>GPQDPYEINLMEELTLKGVTQYYAYVTERQKVHCLNTLFSRLQINQSIIFCNSSQRVELLAKKISQLGYSCFYIHAKMRQEHRNRVFHDFRNGLCRNLVCTDLFTRGIDIQAVNVVINFDFPKLAETYLHRIGRSGRFGHL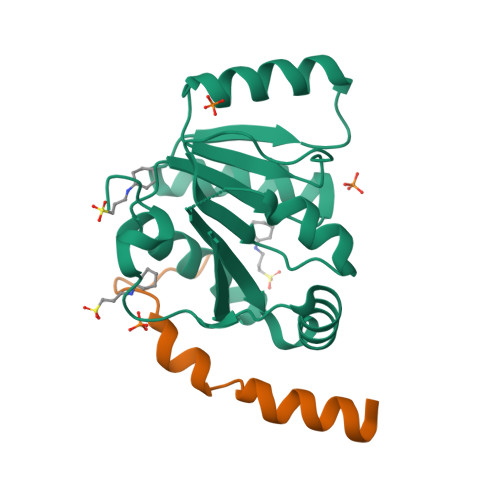GLAINLITYDDRFNLKSIEEQLGTEIKPIPSNIDKSLYVAEYHSEPVEDEKP[2x];>[2x]GPHMADLFGDDIEEIPDTDFDFEGNLALFDKAAVFEEIDTYERR~{N}-cyclobutyl-3-(6-ethanoylpyrrolo[1,2-a]pyrimidin-8-yl)-4-methoxy-benzamide 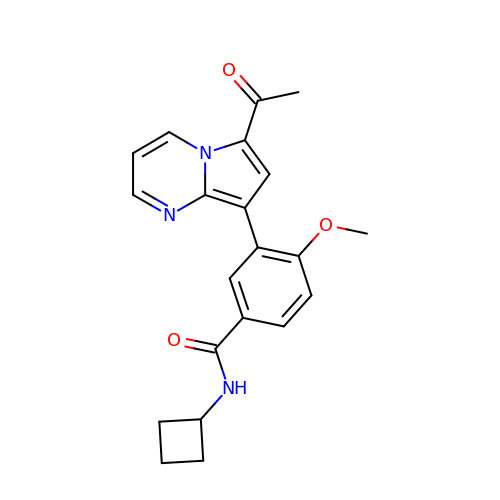| C21 H21 N3 O3 | ZVDRWJICVNPHJL-UHFFFAOYSA-N>[12x]MIANENIQ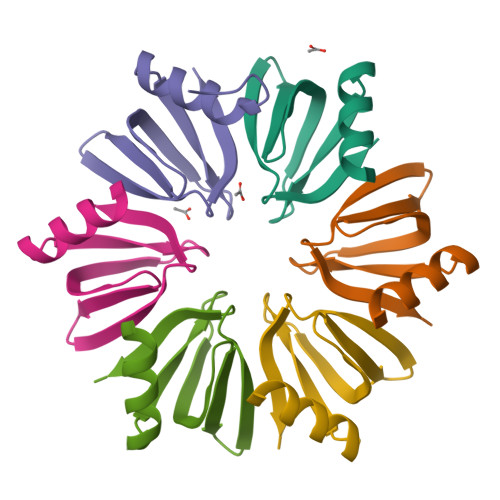DKALENFKANQTEVTVFFLNGFQMKGVIEEYDKYVVSLNSQGKQHLIYKHAISTYTVETEGQASTESEE> MPAAAPG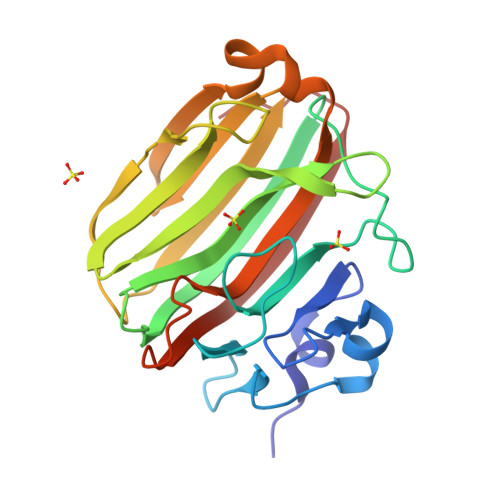KNFDLSHWKLQLPDANTTEISSANLGLGYTSQYFYTDTDGAMTFWAPTTGGTTANSSYPRSELREMLDPSNSKVNWGWQGTHTMKLSGKTVQLPSSGKIIVAQIHGIMDDGTNAPPLVKAVFQDGQLDMQVKQNSDGTGSDVHNYFTGIKLGDLYNMEIRVTDGVAYVTMNGDTRSVDFVGKDAGWKNLKYYFKAGNYVQDNTSTGGSAIAKLYSLSVSHSNLEHHHHHH Acetylcholinesterase inhibitors were introduced for the symptomatic treatment of Alzheimer’s disease (AD). The X-ray crystal structures of Torpedo californica AChE in complex with two novel rigid DNP-like analogs, compounds 1 and 2, have been determined. Compounds 1 and 2 are rigid DNP derivatives synthesized by using an innovative eco-friendly synthetic procedure. Both molecules have been selected as promising candidates for the development of drugs with dual activity on AChE and BACE-1.40 The C–C double bond that in both ligands links the indanone core to the N-benzyl piperidine moiety lower the flexibility of the molecules compared to DNP. The N-benzylpiperidine moiety adopts an almost identical position/orientation within the enzyme catalytic gorge in the crystal structures of the three TcAChE–ligand complexes.

The ring nitrogen is engaged in an in-line H-bond with water W850 in TcAChE-1 and W750 in TcAChE-2. The carbonyl function on the indanone is not in direct contact with the protein, but in the TcAChE–DNP and TcAChE-1 complexes, water molecules W1254 and W708, respectively, appear to make a structurally conserved water-bridged contact with the main chain NH of Phe288. The average distances between the closest indanone and Trp indole aromatic carbons are 4.1 Å and 4.2 Å in TcAChE-1 and in TcAChE-2, respectively, while the same distance averages to 3.7 Å in TcAChE-DNP. Although 1 and 2 share a similar interaction with the TcAChE active site, the presence of a second methoxy substituent on the indanone moiety of 1, as in DNP, allows a better stacking against Trp279 accounting therefore for its slightly higher inhibitory potency compared to 2, being the Ki values of 11.12 ± 2.88 nM versus 29.86 ± 1.12 nM. In more detail, the methoxy substituent at position 5 of the indanone ring of the 5,6-dimethoxy compound 1 stacks on the benzene ring of Trp279 at a distance of 3.9 Å. The binding of 1 displaces 8 of the conserved water molecules (W742, W749, W795, W628, W625, W678, W679, W767) in the native not inhibited TcAChE crystal structure and one new molecule (W874) is stabilized. Overall, according to the crystallographic structures, the binding of 1 displaces from the TcAChE gorge a larger number of solvent molecule than DNP, i.e. 7 versus 3. The rigidity introduced by the double C–C bond compels the indanone moiety of 1 and 2 to a somewhat less effective interaction with the peripheral anionic binding site residue Trp279 at the entrance of the catalytic gorge if compared to the TcAChE–DNP complex.

> DDHSELLVNTKSGKVMGTRVPVLSSHISAFLGIPFAEPPVGNMRFRRPEPKKPWSGVWNASTYPNNCQQYVDEQFPGFSGSEMWNPNREMSEDCLYLNIWVPSPRPKSTTVMVWIYGGGFYSGSSTLDVYNGKYLAYTEEVVLVSLSYRVGAFGFLALHGSQEAPGNVGLLDQRMALQWVHDNIQFFGGDPKTVTIFGESAGGASVGMHILSPGSRDLFRRAILQSGSPNCPWASVSVAEGRRRAVELGRNLNCNLNSDEELIHCLREKKPQELIDVEWNVLPFDSIFRFSFVPVIDGEFFPTSLESMLNSGNFKKTQILLGVNKDEGSFFLLYGAPGFSKDSESKISREDFMSGVKLSVPHANDLGLDAVTLQYTDWMDDNNGIKNRDGLDDIVGDHNVICPLMHFVNKYTKFGNGTYLYFFNHRASNLVWPEWMGVIHGYEIEFVFGLPLVKELNYTAEEEALSRRIMHYWATFAKTGNPNEPHSQESKWPLFTTKEQKFIDLNTEPMKVHQRLRVQMCVFWNQFLPKLLNATACDGELSS4-(2-[(5-fluoro-6-methoxypyridin-3-yl)amino]-5-{(1R)-1-[4-(methylsulfonyl)piperazin-1-yl]ethyl}pyridin-3-yl)-6-methyl-1,3,5-triazin-2-amine 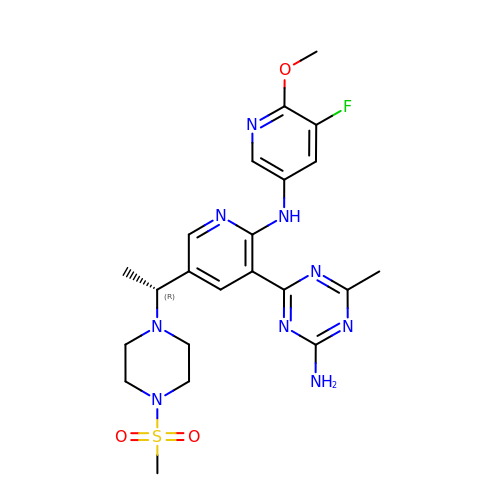| C22 H28 F N9 O3 S | KUGIFHQBIIHRIZ-CYBMUJFWSA-N Activation of the replicative Mcm2-7 helicase by loading GINS and Cdc45 is crucial for replication origin firing, and as such for faithful genetic inheritance. Our biochemical and structural studies demonstrate that the helicase activator GINS interacts with TopBP1 through two separate binding surfaces, the first involving a stretch of highly conserved amino acids in the TopBP1-GINI region, the second a surface on TopBP1-BRCT4. The two surfaces bind to opposite ends of the A domain of the GINS subunit Psf1. Mutation analysis reveals that either surface is individually able to support TopBP1-GINS interaction, albeit with reduced affinity.

With all this information in hand, we could improve the resolution of our cryo-EM data, using an alternative GINS-expression construct, which omits the Psf1-B domain, and served to improve detail around the predicted interaction region. The resultant map showed a volume of extra density that allowed a short helical element to be incorporated into our model, consistent with the AlphaFold2-Multimer predictions. The hydrophobic side of the amphipathic GINI-core helix can be seen to pack across two helices of the Psf1-A domain, making interactions with the side chains of Leu490 and Leu491 of the GINI region and Val47, Lys51, Ile59, Ile62, Lys63 and His66 of Psf1. In addition, the side chain of Tyr494 in the GINI region is inserted into a small pocket on the surface of Psf1 formed by Tyr40, Asn43 and Leu69 with the hydroxyl group picking up a hydrogen bond with the side chain of His66. The GINS interaction surface in BRCT4 consists of residues found at the edge of the central four-stranded β-sheet, with additional interactions made by residues in the loops connecting the strands, including amino acids in the variant region between strands β3 and β4. Together, TopBP1-BRCT4 binds to the A domain of Psf1 and involves the linker region located towards the B domain. To our knowledge, this represents a novel mode for a BRCT domain-mediated interaction. In BRCT4, the interaction surface involves a region around beta strands β3 and β4. This region diverts from the canonical BRCT fold in that it lacks an alpha helix (α2)44 as if to create space for GINS binding. TopBP1 residues Val590, Thr606 and Val610 appeared to be involved in the interface, providing a series of direct hydrophobic interactions with the side chains of Trp92 and Ile97 in Psf1. Consistent with published Y2H experiments, our structural data indicate that the GINI core helix region interacts with both Psf1 and Psf3, at a position close to the distal end of the Psf1 A domain, whereas BRCT4 interacts with both the base of the Psf1-A domain and the linker that connects it to the B domain.

> MFCEKAMELIRELHRAPEGQLPAFNEDGLRQVLEEMKALYEQNQSDVNEAKSGGRSDLIPTIKFRHCSLLRNRRCTVAYLYDRLLRIRALRWEYGSILPNALRFHMAAEEMEWFNNYKRSLATYMRSLGGDEGLDITQDMKPPKSLYIEVR;> MDAAEVEFLAEKELVTIIPNFSLDKIYLIGGDLGPFNPGLPVEVPLWLAINLKQRQKCRLLPPEWMDVEKLEKMRDHERKEETFTPMPSPYYMELTKLLLNHASDNIPKADEIRTLVKDMWDTRIAKLRVSADSFVRQQEAHAKLDNLTLMEINTSGTFLTQALNHMYKLRTNLQPLESTQSQDF;> MSEAYFRVESGALGPEENFLSLDDILMSHEKLPVRTETAMPRLGAFFLERSAGAETDNAVPQGSKLELPLWLAKGLFDNKRRILSVELPKIYQEGWRTVFSADPNVVDLHKMGPHFYGFGSQLLHFDSPENADISQSLLQTFIGRFRRIMDSSQNAYNEDTSALVARLDEMERGLFQTGQKGLNDFQCWEKGQASQITASNLVQNYKKRKFTDMED;> MHHHHHHGRMDYKDDDDKADYKDDDDKADYKDDDDKGRPMTEEVDFLGQDSDGGSEEVVLTPAELIERLEQAWMNEKFAPELLESKPEIVECVMEQLEHMEENLRRAKREDLKVSIHQMEMERIRYVLSSYLRCRLMKIEKFFPHVLEKEKTRPEGEPSSLSPEELAFAREFMANTESYLKNVALKHMPPNLQKVDLFRAVPKPDLDSYVFLRVRERQENILVEPDTDEQRDYVIDLEKGSQHLIRYKTIAPLVASGAVQLI;> MGSHHHHHHGSLEVLFQGPHMASNSLNSKLEPTLENLENLDVSAFQAPEDLLDGCRIYLCGFSGRKLDKLRRLINSGGGVRFNQLNEDVTHVIVGDYDDELKQFWNKSAHRPHVVGAKWLLECFSKGYMLSEEPYIHANYQPVEIPVSHQPESKAALLKKKNSSFSKKDFAPSEKHEQADEDLLSQYENGSSTVVEAKTSEARPFNDSTHAEPLNDSTHISLQEENQSSVSHCVPDVSTITEEGLFSQKSFLVLGFSNENESNIANIIKENAGKIMSLLSRTVADYAVVPLLGCEVEATVGEVVTNTWLVTCIDYQTLFDPKSNPLFTPVPVMTGMTPLEDCVISFSQCAGAEKESLTFLANLLGASVQEYFVRKSNAKKGMFASTHLILKERGGSKYEAAKKWNLPAVTIAWLLETARTGKRADESHFLIENSTKEERSLETEITNGINLNSDTAEHPRRAWSHPQFEK> QTADGRVGLVPVNSYVTLETDDLDTDEHPVTDAGTVALEPGESAPIVRYDLGQPAAVYAVGATDEANVEYELKVNNSKTVGG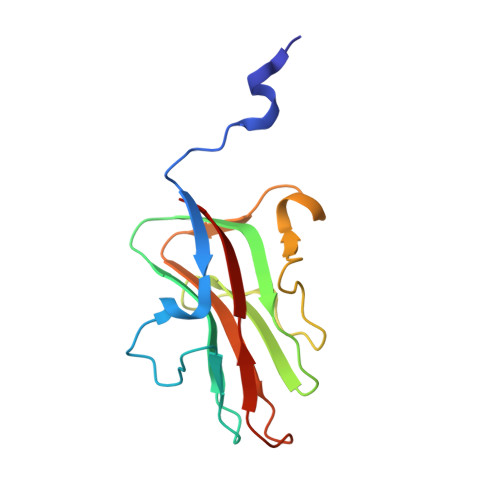RTNSPLGVLNTPFSFVEKLGGAIPCETAATYWAHYSSDATGTVELAGRMHIEV Histone deacetylase complexes remove histone acetylation, thereby repressing transcription and regulating the transcriptional output of each gene. In order to address this, we reconstituted a recombinant version of the human SIN3B complex, composed of the subunits SIN3B isoform 2, HDAC2 (hereafter named HDAC for simplicity), PHF12 and MORF4L1, expressed in the baculovirus/insect cell system. Remarkably, SIN3B encircles the deacetylase and contacts its allosteric basic patch thereby stimulating catalysis. A SIN3B loop inserts into the catalytic tunnel, rearranges to accommodate the acetyl-lysine moiety, and stabilises the substrate for specific deacetylation, which is guided by a substrate receptor subunit.

In conclusion, SIN3B, HDAC, PHF12 and MORF4L1 interact with a 1:1:1:1 stoichiometry to form a V-shaped complex where the SIN3BCTD and substrate recognition module form two arms at the top, the SIN3BHID at the bottom, the HDAC is in the centre, and the SIN3BPAH3 connects the two arms in such a way that the HDAC is completely encircled by the SIN3B subunits. In the SIN3B complex, an additional histone recognition module sits on top of SIN3BMD and HDAC, and includes the MRG domain of MORF4L1, which interacts with the PHF12SID1, and the first PHD domain of PHF12 (PHD1). Strikingly, PHF12PHD1 recognises a composite interface formed by the MORF4L1 MRG domain interacting with the PHF12SID1 as also supported by our XL-MS data. The MRG:SID1:PHD1 ternary assembly form the histone recognition module (or substrate receptor) of SIN3B. Within this structure the PHF12PHD1 is located on top of the active site of the HDAC, suggesting that this domain could recruit the histone tail substrate to the enzyme. In conclusion, our data suggests that PHF12PHD1 and not PHF12PHD2 can deliver the histone H3 substrate to the HDAC active site.

> MAHAGGGSGGSGAGGPAGRGLSGARWGRSGSAGHEKLPVHVEDALTYLDQVKIRFGSDPATYNGFLEIMKEFKSQSIDTPGVIRRVSQLFHEHPDLIVGFNAFLPLGYRIDIPKNGKLNIQSPLTSQENSHNHGDGAEDFKQQVPYKEDKPQVPLESDSVEFNNAISYVNKIKTRFLDHPEIYRSFLEILHTYQKEQLNTRGRPFRGMSEEEVFTEVANLFRGQEDLLSEFGQFLPEAKRSLFTGNGPCEMHSVQKNEHDKTPEHSRKRSRPSLLRPVSAPAKKKMKLRGTKDLSIAAVGKYGTLQEFSFFDKVRRVLKSQEVYENFLRCIALFNQELVSGSELLQLVSPFLGKFPELFAQFKSFLGVKELSFAPPMSDRSGDGISREIDYASCKRIGSSYRALPKTYQQPKCSGRTAICKEVLNDTWVSFPSWSEDSTFVSSKKTPYEEQLHRCEDERFELDVVLETNLATIRVLESVQKKLSRMAPEDQEKFRLDDSLGGTSEVIQRRAIYRIYGDKAPEIIESLKKNPVTAVPVVLKRLKAKEEEWREAQQGFNKIWREQYEKAYLKSLDHQAVNFKQNDTKALRSKSLLNEIESVYDEHQEQHSEGRSAPSSEPHLIFVYEDRQILEDAAALISYYVKRQPAIQKEDQGTIHQLLHQFVPSLFFSQQLDLGASEESADEDRDSPQGQTTDPSERKKPAPGPHSSPPEEKGAFGDAPATEQPPLPPPAPHKPLDDVYSLFFANNNWYFFLRLHQTLCSRLLKIYRQAQKQLLEYRTEKEREKLLCEGRREKGSDPAMELRLKQPSEVELEEYYPAFLDMVRSLLEGSIDPTQYEDTLREMFTIHAYVGFTMDKLVQNIARQLHHLVSDDVCLKVVELYLNEKKRGAAGGNLSSRCVRAARETSYQWKAERCMADENCFKVMFLQRKGQVIMTIELLDTEEAQTEDPVEVQHLARYVEQYVGTEGASSSPTEGFLLKPVFLQRNLKKFRRRWQSEQARALRGEARSSWKRLVGVESACDVDCRFKLSTHKMVFIVNSEDYMYRRGTLCRAKQVQPLVLLRHHQHFEEWHSRWLEDNVTVEAASLVQDWLMGEEDEDMVPCKTLCETVHVHGLPVTRYRVQYSRRPASP;> MAYSQGGGKKKVCYYYDGDIGNYYYGQGHPMKPHRIRMTHNLLLNYGLYRKMEIYRPHKATAEEMTKYHSDEYIKFLRSIRPDNMSEYSKQMQRFNVGEDCPVFDGLFEFCQLSTGGSVAGAVKLNRQQTDMAVNWAGGLHHAKKSEASGFCYVNDIVLAILELLKYHQRVLYIDIDIHHGDGVEEAFYTTDRVMTVSFHKYGEYFPGTGDLRDIGAGKGKYYAVNFPMRDGIDDESYGQIFKPIISKVMEMYQPSAVVLQCGADSLSGDRLGCFNLTVKGHAKCVEVVKTFNLPLLMLGGGGYTIRNVARCWTYETAVALDCEIPNELPYNDYFEYFGPDFKLHISPSNMTNQNTPEYMEKIKQRLFENLRMLPHAPGVQMQAIPEDAVHEDSGDEDGEDPDKRISIRASDKRIACDEEFSDSEDEGEGGRRNVADHKKGAKKARIEEDKKETEDKKTDVKEEDKSKDNSGEKTDTKGTKSEQLSNP;> MWEKMETKTIVYDLDTSGGLMEQIQALLAPPKTDEAEKRSRKPEKEPRRSGRATNHDSCDSCKEGGDLLCCDHCPAAFHLQCCNPPLSEEMLPPGEWMCHRCTVRRKKREQKKELGHVNGLVDKSGKRTTSPSSDTDLLDRSASKTELKAIAHARILERRASRPGTPTSSASTETPTSEQNDVDEDIIDVDEEPVAAEPDYVQPQLRRPFELLIAAAMERNPTQFQLPNELTCTTALPGSSKRRRKEETTGKNVKKTQHELDHNGLVPLPVKVCFTCNRSCRVAPLIQCDYCPLLFHMDCLEPPLTAMPLGRWMCPNHIEHVVLNQKNMTLSNRCQVFDRFQDTVSQHVVKVDFLNRIHKKHPPNRRVLQSVKRRSLKVPDAIKSQYQFPPPLIAPAAIRDGELICNGIPEESQMHLLNSEHLATQAEQQEWLCSVVALQCSILKHLSAKQMPSHWDSEQTEKADIKPVIVTDSSVTTSLQTADKTPTPSHYPLSCPSGISTQNSLSCSPPHQSPALEDIGCSSCAEKSKKTPCGTANGPVNTEVKANGPHLYSSPTDSTDPRRLPGANTPLPGLSHRQGWPRPLTPPAAGGLQNHTVGIIVKTENATGPSSCPQRSLVPVPSLPPSIPSSCASIENTSTLQRKTVQSQIGPPLTDSRPLGSPPNATRVLTPPQAAGDGILATTANQRFSSPAPSSDGKVSPGTLSIGSALTVPSFPANSTAMVDLTNSLRAFMDVNGEIEINMLDEKLIKFLALQRIHQLFPSRVQPSPGSVGTHQLASGGHHIEVQRKEVQARAVFYPLLGLGGAVNMCYRTLYIGTGADMDVCLTNYGHCNYVSGKHACIFYDENTKHYELLNYSEHGTTVDNVLYSCDFSEKTPPTPPSSIVAKVQSVIRRRRHQKQDEEPSEEAAMMSSQAQGPQRRPCNCKASSSSLIGGSGAGWEGTALLHHGSYIKLGCLQFVFSITEFATKQPKGDASLLQDGVLAEKLSLKPHQGPVLRSNSVP;> MAPKQDPKPKFQEGERVLCFHGPLLYEAKCVKVAIKDKQVKYFIHYSGWNKKSAVRPRRSEKSLKTHEDIVALFPVPEGAPSVHHPLLTSSWDEWVPESRVLKYVDTNLQKQRELQKANQEQYAEGKMRGAAPGKKTSGLQQKNVEVKTKKNKQKTPGNGDGGSTSETPQPPRKKRARVDPTVENEETFMNRVEVKVKIPEELKPWLVDDWDLITRQKQLFYLPAKKNVDSILEDYANYKKSRGNTDNKEYAVNEVVAGIKEYFNVMLGTQLLYKFERPQYAEILADHPDAPMSQVYGAPHLLRLFVRIGAMLAYTPLDEKSLALLLNYLHDFLKYLAKNSATLFSASDYEVAPPEYHRKAV>MGSSHHHHHHSQDHENLYFQGSMGLEKGFTHPTDRVVRLKNMILHAKPYVESERAVLATEAYKENEQLPAIMRRAKVVEKIFNELPVTIRPDELIVGAVTINPRSTEICPEFSYDWVEKEFDTMAHRVADPFIIEKKTADELHQAFKYWPGKTTSSLAASYMSEGTKESMSNGVFTVGNYFFGGIGHVSVDYGKVLKIGFRGIIDEVTRALENLDRSTSDYIKKEQFYNAVILSYQAAINFAHRYAQEASRLAREERDPTRQRELEQIASNCTRVPEYGATTFWEACQTFWFIQSMLQIESSGHSISPGRFDQYMYPYLAADTAISSEFAQELVDCCWIKLNDINKTRDEISAQAFAGYAVFQNLCVGGQ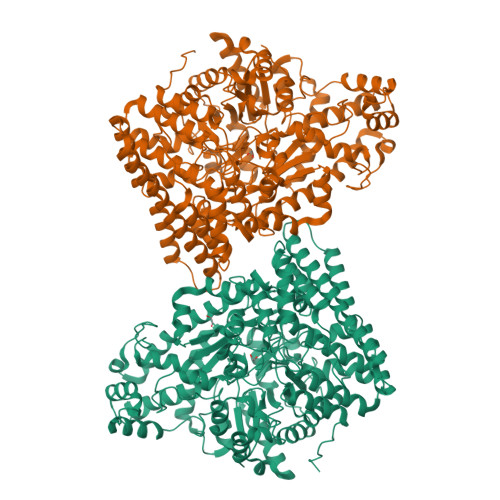TEDGRDATNPLTYMCMEATAHVRLPQPSFSIRVWQGTPDEFLYRACELVRLGLGVPAMYNDEVIIPALQNRGVSLHDARDYCIIGCVEPQAPHRTEGWHDAAFFNVAKVLEITLNNGRSGNKQLGPMTGEMTQYAGMDDFYAAFKKQMAHFVHQLVEACNSVDIAHGERCPLPFLSALVDDCIGRGKSLQEGGAIYNFTGPQAFGIADTGDSVYAIQKQVFEDRRLTLQELKGALDANFGYRSGNPRYEEIRHILENSPCFGNDIDDVDLVARQCALIYCQEVEKYTNPRGGRFQAGIYPVSANVLFGKDVSALPDGRLAKEPLADGVSPRQGKDTLGPTAAANSVAKLDHFIASNGTLYNQKFLPSSLAGEKGLRNFGGLVRNYFDKKGMHVQFNVIDRNTLLEAQKNPQQHQDLVVRVAGYSAQFVVLAKEVQDDIISRTEQQF[4x]>[3x]MFKKLLDNKNLVINPPVFITSILLIVALILTCVLFPEKVGVWFPAAQLAVTSNFGWFFVVTVNVILIFAIYLAFSKFGRIRLGGDDAEPEFTKASWFAMLFSTGMGIGIMFFSIAEPVSHFFNTPRPVDTDIEAAVQAMQFTSLHWGLHAWGIYAMVGLALAFFGFNRKLPMTFRSLFYPFWGERIHGWWGHIIDILSALATVFGLSTSLGLGVIQITAGLEYLYGWEISPMMQAGIILFVIGIATISVFSGLDKGVKILSNANMYIAASFMLLIFILGPTLFIMKGYVENTGAYLANFIDISTWNDTYLGSGWQNVWTIFYWAWWIAWSPFVGSFIARISKGRTVKEFVLGVLIVPGLITLLWMNVFGGSALHTILSGD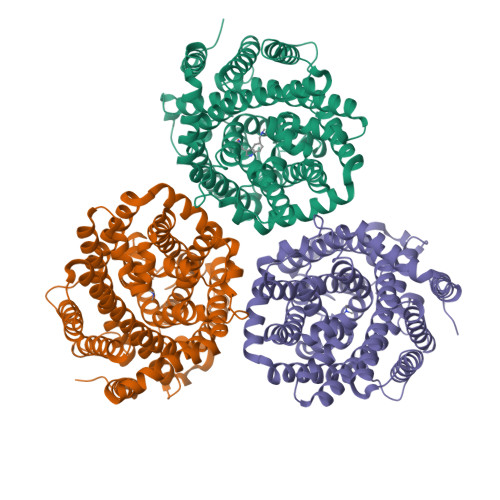VTMIAAVKADVSTALFVFLENFPFTKFLSIVAIILIFSFFITSSDSGSLVVDNITSGSNGESPVWQRVFWSFAQGIIAIVLLWGGGLDALQTAVIITGLPFAVILLVMCYSLQKGLKEELAKSSKKAKSKEEKSYKEIIAELLDEPQSKHHHHHHHHHH Here, we report the three-dimensional structure of a ‘Termamyl’-like α-amylase, the AliC α-amylase from Alicyclobacillus sp. 18711. One particularly important subset of GH13 enzymes are the ‘Termamyl’-like α-amylases, historically named after an enzyme from Bacillus licheniformis. These enzymes typically feature a three-domain ‘A, B, C’ arrangement with a C-terminal β-sheet domain and with domain B being a protrusion from the (β/α)8 fold of domain A. The catalytic centre is placed in domain A, whilst the A–B interface forms the substrate-binding cleft. The fold, as expected, is a canonical three-domain arrangement with the A, B and C domains defined approximately as A, residues 4–104 and 210–397; B, residues 105–209; and C, residues 398–484. A classical Ca2+–Na+–Ca2+ triad is found at the A/B-domain interface.

The complex of AliC with acarbose was solved by molecular replacement, with two molecules of AliC in the asymmetric unit, at a resolution of 2.1 Å. The structure of AliC was determined in the presence of the inhibitor acarbose. As with many (retaining) α-amylase complexes [some examples from the author’s laboratory include those reported in Brzozowski et al., Davies et al., Brzozowski & Davies, Dauter et al. and Offen et al.], the acarbose is observed as a transglycosylated species, here a hexasaccharide which contains two of the acarviosin disaccharide motifs. An initial ligand-bound structure with a transglycosyl­ated acarbose-derived oligosaccharide at a resolution of 2.1 Å revealed a noncovalently linked glucose moiety, hinting at a putative branch-accommodation site around the +2/+3 subsites. Of particular interest to us was the observation of a ‘lone’ ordered glucose moiety that was not covalently linked to the acarbose-derived oligosaccharide in a position that could be indicative of the accommodation of branch points at either the +2 or +3 positions of AliC. An additional isolated glucose molecule, modelled in both α and β anomeric forms (occupancy set at 0.5 for each and in different orientations; omitted from Fig. 1 for clarity), was observed near a potential +3 site. We speculated whether these isolated glucose moieties could provide insight into branch-point recognition. At the time of writing, structural similarity searches using PDBeFold showed that the closest three-dimensional match to AliC is the B. halmapalus α-amylase, with 67% sequence identity and with 479 aligned Cα atoms overlapping with an r.m.s.d. of 0.49 Å (PDBeFold Q score 0.95, Z-score 27.8).

>TFAGDNGTMMQYFEWYLPNDGTLWTKMGSDASHLKSIGITGVWFPPAYKGQSQSDVGYGVYDMYDLGEFNQKGTVRTKYGTKAQLQSAITSLHNNGIQAYGDVVLNHRMGADATETISAVEVNPSNRNQVTSGAYNISAWTDFEFPGRGNTYSSFKWHSYYFDGVDWDQSRQLSGKIYQIQGKAWDWEVDSENGNYDYLMGADIDYDHPDVQTEVKNWGKWFVNTLNLDGVRLDAVKHIKFDYMSSWLSSVKSTTGKSNLFAVGEYWNTSLGALENYENKTNWSMSLFDVPLHMNFQAAANGGGYYDMRNLLNNTMMKNHPIQAVTFVDNHDTEPGQALQSWVSDWFKPLAYATILTRQEGYPCVFYGDYYGIPSQSVSAKSTWLDKQLSARKSYAYGTQHDYLDNQDVIGWTREGDSAHAGSGLATVMSDGPGGSKTMYVGTAHAGQVFKDITGNRTDTVTINSAGNGTFPCNGGSVSIWVKQ[2x]>[4x]AKVN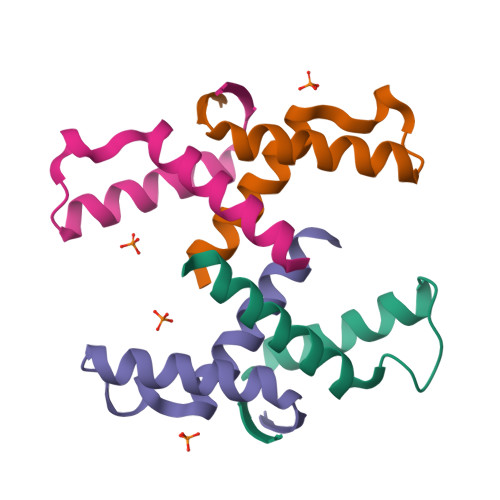LYISNDAYEKINAIIEKRRQEGAREKDVSFSATASMLLELGLRVHEAQM> HHHHHHHHVPEAFLLFSRRADIRRISLETNNNNVAIPLTGVKEASALDFDVTDNRIYWTDISLKTISRAFMNGSALEHVVEFGLDYPEGMAVDWLGKNLYWADTGTNRIEVSKLDGQHRQVLVWKDLDSPRALALDPAEGFMYWTEWGGKPKIDRAAMDGSERTTLVPNVGRANGLTIDYAKRRLYWTDLDTNLIESSNMLGLNREVIADDLPHPFGLTQYQDYIYWTDWSRRSIERANKTSGQNRTIIQGHLDYVMDILVFHSSRQSGWNECASSNGHCSHLCLAVPVGGFVCGCPAHYSL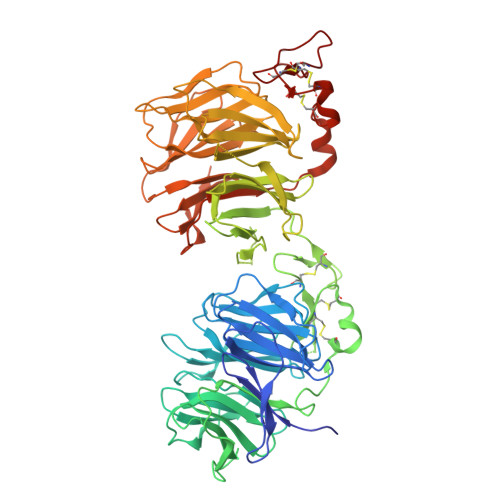NADNRTCSAPTTFLLFSQKSAINRMVIDEQQSPDIILPIHSLRNVRAIDYDPLDKQLYWIDSRQNMIRKAQEDGSQGFTVVVSSVPSQNLEIQPYDLSIDIYSRYIYWTCEATNVINVTRLDGRSVGVVLKGEQDRPRAIVVNPEKGYMYFTNLQERSPKIERAALDGTEREVLFFSGLSKPIALALDSRLGKLFWADSDLRRIESSDLSGANRIVLEDSNILQPVGLTVFENWLYWIDKQQQMIEKIDMTGREGRTKVQARIAQLSDIHAVKELNLQEYRQHPCAQDNGGCSHICLVKGDGTTRCSCPMHLVLLQDELSC(S)-(ALPHA)-METHYL-4-CARBOXYPHENYLGLYCINE | C10 H11 N O4 | 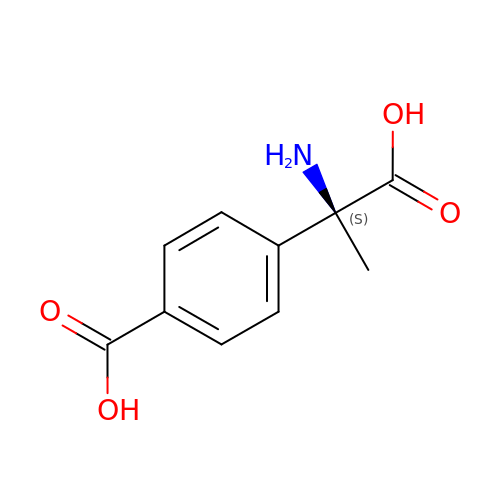DNCAZYRLRMTVSF-JTQLQIEISA-N> VI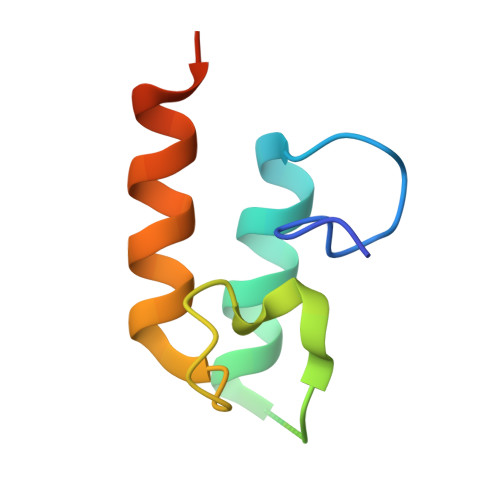VYGDYNNDGNVDALDFAGLKKYIMAADHAYVKNLDVNLDNEVNSTDLAILKKYLLGMVSKLPSN> MEAAHSKSTEECLAYFGVSETTGLTPDQVKRHLEKYGHNELPAEEGKSLWELVIEQFEDLLVRILLLAACISFVLAWFEEGEETITAFVEPFVILLILIANAIVGVWQERNAENAIEALKEYEPEMGKVYRADRKSVQRIKARDIVPGDIVEVAVGDKVPADIRILSIKSTTLRVDQSILTGESVSVIKHTEPVPDPRAVNQDKKNMLFSGTNIAAGKALGIVATTGVSTEIGKIRDQMAATEQDKTPLQQKLDEFGEQLSKVISLICVAVWLINIGHFNDPVHGGSWIRGAIYYFKIAVALAVAAIPEGLPAVITTCLALGTRRMAKKNAIVRSLPSVETLGCTSVICSDKTGTLTTNQMSVCKMFIIDKVDGDFCSLNEFSITGSTYAPEGEVLKNDKPIRSGQFDGLVELATICALCNDSSLDFNETKGVYEKVGEATETALTTLVEKMNVFNTEVRNLSKVERANACNSVIRQLMKKEFTLEFSRDRKSMSVYCSPAKSSRAAVGNKMFVKGAPEGVIDRCNYVRVGTTRVPMTGPVKEKILSVIKEWGTGRDTLRCLALATRDTPPKREEMVLDDSSRFMEYETDLTFVGVVGMLDPPRKEVMGSIQLCRDAGIRVIMITGDNKGTAIAICRRIGIFGENEEVADRAYTGREFDDLPLAEQREACRRACCFARVEPSHKSKIVEYLQSYDEITAMTGDGVNDAPALKKAEIGIAMGSGTAVAKTASEMVLADDNFSTIVAAVEEGRAIYNNMKQFIRYLISSNVGEVVCIFLTAALGLPEALIPVQLLWVNLVTDGLPATALGFNPPDLDIMDRPP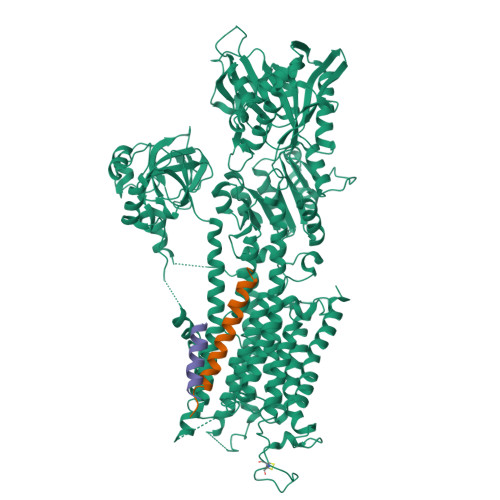RSPKEPLISGWLFFRYMAIGGYVGAATVGAAAWWFMYAEDGPGVTYHQLTHFMQCTEDHPHFEGLDCEIFEAPEPMTMALSVLVTIEMCNALNSLSENQSLMRMPPWVNIWLLGSICLSMSLHFLILYVDPLPMIFKLKALDLTQWLMVLKISLPVIGLDEILKFIARNYLEG;> MDKVQYLTRSAIRRASTIEMPQQARQNLQNLFINFCLILICLLLICIIVM> MSLVTATAAQRIALRNTATNLSEQTQVYAQSATAPTAAEAAIVQPYIDAAQAAITAVGAGGATV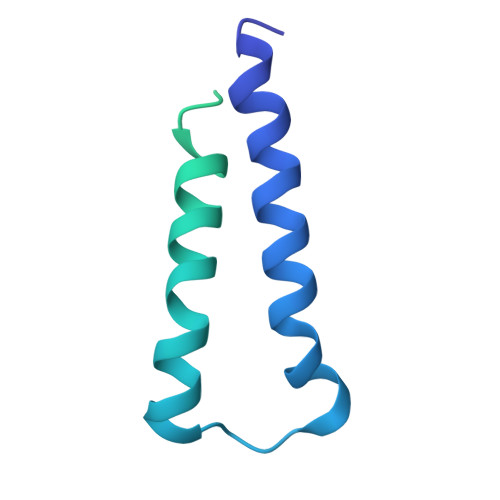ANGATVAVVNSASADSHNATATVTGTTLTNVKLAATVAFVDNADTITVQNSAGTAVAGTHTATVAAGVISNVKLAATIAPVASGLALTGVTPTGTYTNTVTFTVAAGVITAIVLS>AHCIGITDRDFIEGVHGGTWVSATLEQDKCVTVMAPDKPSLDISLETVAIDGPAEARKVCYNAVLTHVKINDKCPSTGEAHLAEENEGDNACKRTYSDRGWGNGCGLFGKGSIVACAKFTCAKSMSLFEVDQTKIQYVIRAQLHVGAKQENWNTDIKTLKFDALSGSQEAEFTGYGKATLECQVQTAVDFGNSYIAEMEKESWIVDRQWAQDLTLPWQSGSGGVWREMHHLVEFEPPHAATIRVLALGNQEGSLKTALTG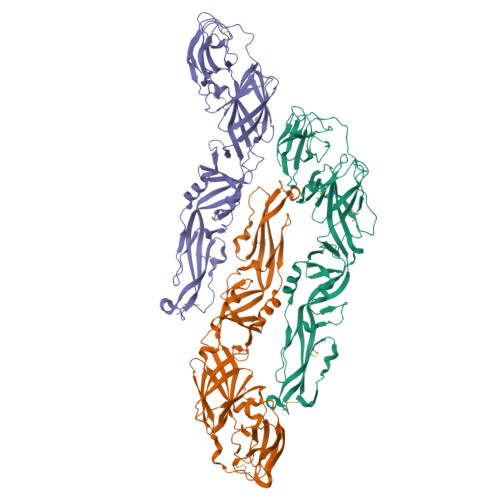AMRVTKDTNDNNLYKLHGGHVSCRVKLSALTLKGTSYKICTDKMFFVKNPTDTGHGTVVMQVKVSKGAPCRIPVIVADDLTAAINKGILVTVNPIASTNDDEVLIEVNPPFGDSYIIVGRGDSRLTYQWHK[3x]> MGSSHHHHHHSQDPNSHMKETPLSNCERRFLLRAIEEKKRLDGRQTYDYRNIRI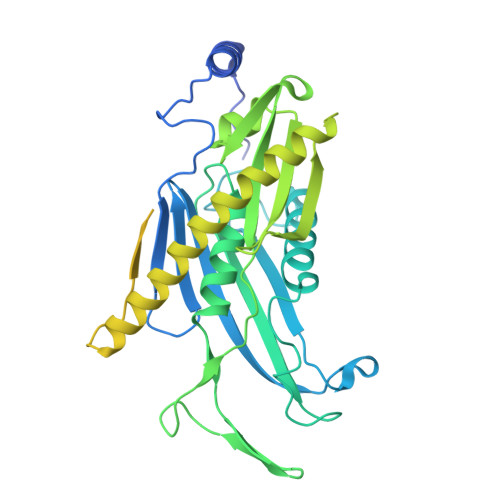SFGTDYGCCIVELGKTRVLGQVSCELVSPKLNRATEGILFFNLELSQMAAPAFEPGRQSDLLVKLNRLMERCLRNSKCIDTESLCVVAGEKVWQIRVDLHLLNHDGNIIDAASIAAIVALCHFRRPDVSVQGDEVTLYTPEERDPVPLSIHHMPICVSFAFFQQGTYLLVDPNEREERVMDGLLVIAMNKHREICTIQSSGGIMLLKDQVLRCSKIAGVKVAEITELILKALENDQKVRKEGGKFGFAESIANQRITAFKMEKAPIDTSDVEEKAEEIIAEAEPPSEVVSTPVLWTPGTAQIGEGVENSWGDLEDSEKEDDEGGGDQAIILDGIKMDTGVEVSDIGSQELGFHHVGQTGLEFLTSDAPIILSDSEEEEMIILEPDKNPKKIRTQTTSAKQEKAPSKKPVKRRKKKRAAN> DLTVKEKEELIEEWQPEPLVPPVPKDHPALNYNIVSGPPSHKTVVNGKECINFASFNFLGLLDNPRVKAAALASLKKYGVGTCGPRGFYGTFDVHLDLEDRLAKFMKTEEAIIYSYGFATIASAIPAYSKRGDIVFVDRAACFAIQKGLQASRSDIKLFKHNDMADLERLLKEQEIEDQKNPRKARVTRRFIVVEGLYMNTGTICPLPELVKLKYKYKARIFLEESLSFGVLGEHGRGVTEHYGINIDDIDLISANMENALASIGGFCCGRSFVIDHQRLSGQGYCFSASLPPLLAAAAIEALNIMEENPGIFAVLKEKCGQIHKALQGISGLKVVGESLSPAFHLQLEESTGSREQDVRLLQEIVDQCMNRSIALTQARYLEKEEKCLPPPSIRVVVTVEQTEEELERAASTIKEVAQAVLL;> MRPEPGGCCCRRTVRANGCVANGEVRNGYVRSSAAAAAAAAAGQIHHVTQNGGLYKRPFNEAFEETPMLVAVLTYVGYGVLTLFGYLRDFLRYWRIEKCHHATEREEQKDFVSLYQDFENFYTRNLYMRIRDNWNRPICSVPGARVDIMERQSHDYNWSFKYTGNIIKGVINMGSYNYLGFARNTGSCQEAAAKVLEEYGAGVCSTRQEIGNLDKHEELEELVARFLGVEAAMAYGMGFATNSMNIPALVGKGCLILSDELNHASLVLGARLSGATIRIFKHNNMQSLEKLLKDAIVYGQPRTRRPWKKILILVEGIYSMEGSIVRLPEVIALKKKYKAYLYLDEAHSIGALGPTGRGVVEYFGLDPEDVDVMMGTFTKSFGASGGYIGGKKELIDYLRTHSHSAVYATSLSPPVVEQIITSMKCIMGQDGTSLGKECVQQLAENTRYFRRRLKEMGFIIYGNEDSPVVPLMLYMPAKIGAFGREMLKRNIGVVVVGFPATPIIESRARFCLSAAHTKEILDTALKEIDEVGDLLQLKYSRHRLVPLLDRPFDETTYEETED;> MADYKDDDDKSGPDEVDASGRMAGMALARAWKQMSWFYYQYLLVTALYMLEPWERTVFNSMLVSIVGMALYTGYVFMPQHIMAILHYFEIVQ;> MNVGTAHSEVNPATRVMNSRGIWLSYVLAIGLLHIVLLSIPFVSVPVVWTLTNLIHNMGMYIFLHTVKGTPFETPDQGKARLLTHWEQMDYGVQFTASRKFLTITPIVLYFLTSFYTKYDQIHFVLNTVSLMSVLIPKLPQLHGVRIFGINKY;> MATATEQWVLVEMVQALYEAPAYHLILEGILILWIIRLLFSKTYKLQERS

The ORM/ORMDL family proteins function as regulatory subunits of the serine palmitoyltransferase (SPT) complex, which is the initiating and rate-limiting enzyme in sphingolipid biosynthesis. In humans, the heterotrimeric SPT core enzymatic complex, composed of SPTLC1, SPTLC2 or SPTLC3, and SPTssa or SPTssb, catalyzes the first and rate-limiting step of de novo sphingolipid biosynthesis by condensation of serine and palmitoyl-CoA to generate 3-keto-dihydrosphingosine (3-KDS). As a critical mechanism for the homeostatic regulation of sphingolipid production, SPT activity is inhibited in response to elevated cellular sphingolipid levels in an ORM/ORMDL-dependent manner. In this work, we demonstrate that ceramide binds directly with and inhibits the human SPT-ORMDL complexes, a process that is important for establishing cellular sphingolipid homeostasis.

To elucidate the molecular defects of the ceramide binding mutant, we then determined the structure of the SPT-ORMDL3 variant containing ORMDL3-N13A mutation at an overall resolution of 2.9 Å for the monomeric complex. Structural comparison of this ceramide binding mutant with WT SPT-ORMDL3 reveals little conformational variations, except for two evident local structural differences. Firstly, the ceramide-like density basically disappeared in the ORMDL3-N13A mutant, corroborating the largely disrupted ceramide binding by this point mutation. Consistent with this, the purified ORMDL3-N13A mutant demonstrated a decrease in ceramide enrichment of approximately 30% compared to the WT complex. Secondly, the N-terminal 10 residues of ORMDL3 became flexible in the ORMDL3-N13A mutant, explaining why this ceramide binding mutant is no longer able to suppress SPT activity efficiently. Several residues that contributed to the intramolecular polar interactions at the ORMDL3 N-terminus in WT SPT-ORMDL3 structure, such as Asn11, Arg15, and Tyr91, exhibited apparent structural shifts in the ORMDL3-N13A mutant. We suggest that ceramide binding might trigger the conformational changes of Asn13 and the adjacent residues in ORMDL3, which could induce and lock the ORMDL3 N-terminus into an inhibitory conformation. Although the SPT-ORMDL3 (ORMDL3-N13A) variant displayed a similar Vmax value to that of the WT SPT complex, the Khalf value of this variant toward palmitoyl-CoA was nearly two times as high as that of the WT SPT complex. This suggests that in the absence of ceramide binding, ORMDL3 can still inhibit SPT by reducing the affinity of SPT for palmitoyl-CoA substrate. The Asn13 in ORMDL is critical for ceramide binding.>GGUGGUGAAGUCGCUGG[2x];>CAGCGXCACACCACCC[2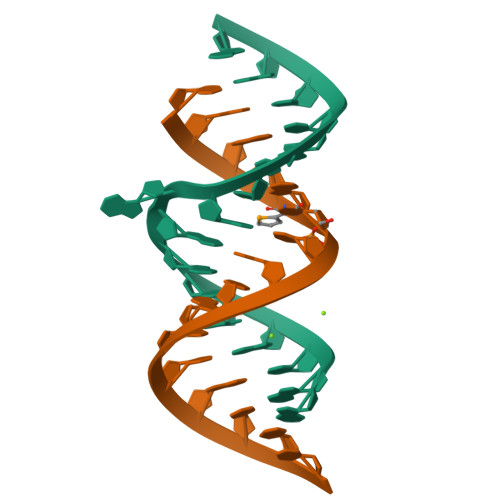x]>MGHHHHHHSSENLYFQGHMASMACRTRFAPSPTGYLHIGGARTALYCWLEARRRGGQFVLRIEDTDRQRSTQAAIDAILEAMQWLGLGYDEGPIYQTQRVARYQEVAEQLLAQGKAYYAYETREELDAMREAAMAKQEKPRYDGAAREQNLPYRDDPNRVIRFKNPIGGTVVFDDLIKGRIEIANSELDDMVIFRPDGLPTYNFAVVVDDWDMGITEVIRGDDHINNTPRQINIYAALGAPVPKFAHMPMILDEQGTKLSKRTGAADVMQYKDAGYLPHALINYLARLGWSHGDQELFTPQELLDLFDVKDVNSKAARLDMAKLGWVNQHYLKTDDPASIAPQLEYQLAKLGVDLAAGPAAADVVVALRERVHTLKEMAEKAVVWYQPLETYDAAAVMKHLKLGAEVPLGKARELLAAVDQWSVDSVSAALHDAAAALELGMGK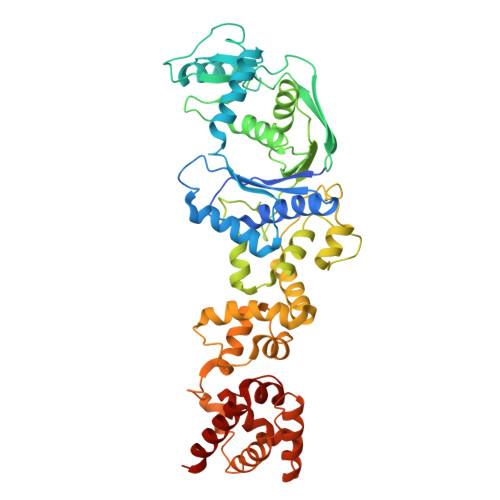VAQPLRVAITGTQVSPDISQTVYLAGREGALKRIDAALTKIGAA[6x]>LVPRGSHMMKTLSLQSRAKTTALKQPKEIFAFARDIDGEFVYDQKIVKDENVSYYYLPDSKIDGSIDLQAGYAKFKKIPEEKNMSDMKCLLTALTKYEQEHNNGEKVNVDIITYRGLMTKLLALPYNLNDPVDLNVLAYDGQLFINSDEEIELARRKEEDEHKQQSMTPEKYDHMKRCEFSGYKFEAIATLPKPWADCSRQQIDKRGKKMVNNYEQYISVIKTGIGEAKMLLAGEVDCVWDYIPEDGKDVLSHYMELKTTRILESNGQVVNFEKKLFKTWAQCFLMGIRKVVYGFRD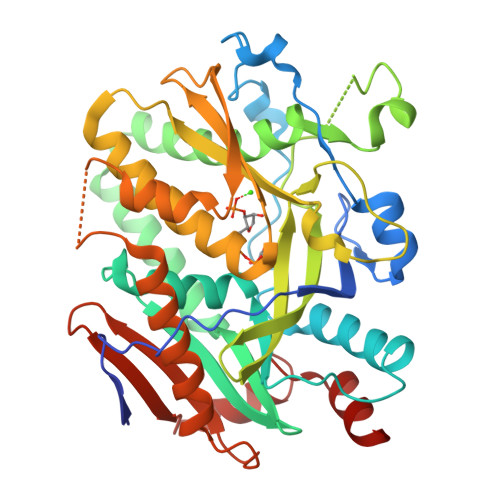DSFFLRDVELYKTEEIPLLIKNNALTENKSGGKINCTTALKWYGAVIEWLLQEIPRDDTSKAYRVSFDPSTRTFTLRELMGNENSRLRNGEMLTSEFKQWRESI[4x]>[8x]MEEENIVNGDRPRDLVFPGTAGLQLYQSLYKYSYITDGIIDAHTNEVISYAQIFETSCRLAVSLEKYGLDHNNVVAICSENNIHFFGPLIAALYQGIPMATSNDMYTEREMIGHLNISKPCLMFCSKKSLPFILKVQKHLDFLKKVIVIDSMYDINGVECVFSFVSRYTDHAFDPVKFNPKEFDPLERTALIMTSSGTTGLPKGVVISHRSITIRFVHSSDPIYGTRIAPDTSILAIAPFHHAFGLFTALAYFPVGLKIVMVKKFEGEFFLKTIQNYKIASIVVPPPIMVYLAKS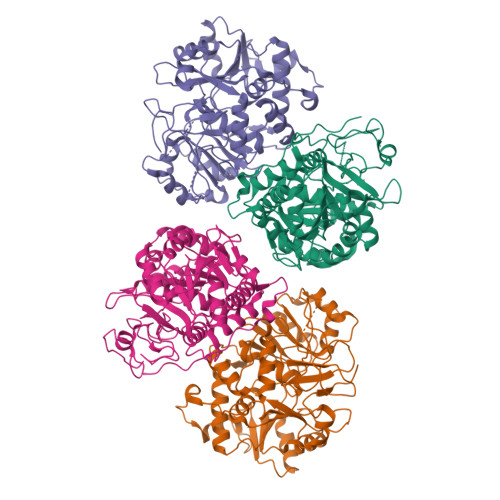PLVDEYNLSSLTEIACGGSPLGRDIADKVAKRLKVHGILQGYGLTETCSALILSPNDRELKKGAIGTPMPYVQVKVIDINTGKALGPREKGEICFKSQMLMKGYHNNPQATRDALDKDGWLHTGDLGYYDEDRFIYVVDRLKELIKYKGYQVAPAELENLLLQHPNISDAGVIGIPDEFAGQLPSACVVLEPGKTMTEKEVQDYIAELVTTTKHLRGGVVFIDSIPKGPTGKLMRNELRAIFAREQAKSKL> MPELTRRHALGAAAALAAVAGTQALAAPSASAAGHHGGPQPFDEVYQGRRIEGRATGGGHHHGSGYG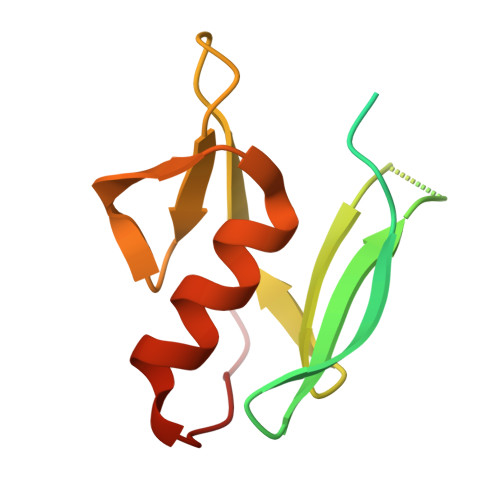VFIDGMELHVMQNVDGSWISVVSHYDPVATPRAAARAAVVELQGAPLVPFN> AEIYNKDGNKVDLYGCAVGLHYFSKGNGENSYGGNGDMTYARLGFKGETQINSDLTGYGQWEYNFQGNNSEGADAQTGNKTRLAFAGLKYADVGSFDYGRNYGVVYDALGYTDMLPEFGGDTAYSDDFFVGRVGGVATYRNSNFFGLVDGLNFAVQYLGKNERDTARRSNGDGVGGSISYEYEGFGIVGAYGAADRTNLQEAQPLGNGKKAEQWATGLKYDANNIYLAANYGETRNATPITNKFTNTSGFANKTQDVLLVAQYQFDFGLRPSIAYTKSKAKDVEGIGDVDLVNYFEVGATYYFNKNMS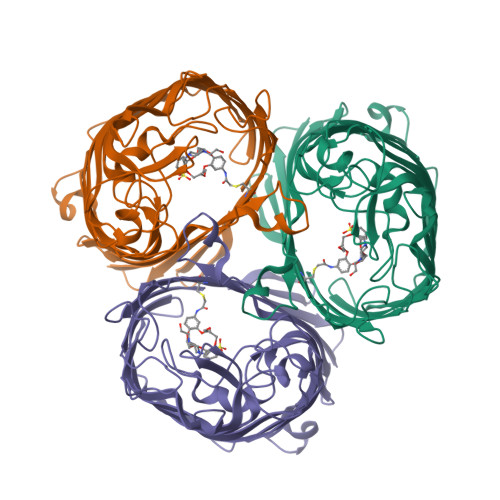TYVDYIINQIDSDNKLGVGSDDTVAVGIVYQF Here we elucidate the structural and molecular determinant(s) of target specificity of histidine vs. lysine in the active site of SETD3. On the substrate-binding surface, the residues are diverse, reflecting the fact that the three enzymes act on three very distinct substrates—the large subunit of Rubisco by LSMT, RelA subunit of nuclear factor NFκB by SETD6, and actin by SETD3—with limited sequence similarity immediately surrounding the methylation target. To facilitate the methyl transfer reaction, SETD3 provides a local environment that promotes deprotonation of the target nitrogen N3 of histidine (and concomitant protonation of N1). Most (if not all) SAM-dependent MTases use the classic SN2 reaction mechanism, which requires the target nitrogen be in a deprotonated state.

Second, we incubated SETD3 with actin peptide in the presence of a molar excess of SAM (at pH 8.0) and crystallized the post-reactive product complex, i.e., the methylated histidine and SAH. The methyl group at the N3 position of methylhistidine is 3.2 Å away from the sulfur atom of SAH, where the transferable methyl group was attached before the reaction, and makes three weak C–H•••O hydrogen bonds, respectively, with the main chain carbonyl oxygen atoms of Thr252 and Asp274 as well as the hydroxyl oxygen of Tyr312. The methylated imidazole ring is perpendicular to the aromatic ring of Tyr312, and the nitrogen atom N1 is within H-bond distance from the side chain of Asn255. The current configuration of Asn255 appears to serve as a proton acceptor from the protonated N1 (N1–H•••O=C) of methylated H73; and to donate two protons to the main chain carbonyl oxygen atom of Ala268, and to a water molecule (numbered w2). The water (w2), in turn, forms three additional H-bonds with the main chain amide nitrogen atom of Ile270, one of the side chain carboxylate oxygen atoms of Asp274, and the main chain carbonyl oxygen atom of Arg253. This suggests that immediately after methyl transfer, the methylated histidine is positively charged with a protonated N1 (N1-H) and a methylated N3 (N3-CH3) and forms a cation–π interaction with Tyr312. The main difference between the pre-reactive and post-reactive complex structures is that the imidazole ring of methylated His73 rotated away from that of histidine.

>[2x]GPLGSMGKKSRVKTQKSGTGATATVSPKEILNLTSELLQKCSSPAPGPGKEWEEYVQIRTLVEKIRKKQKGLSVTFDGKREDYFPDLMKWASENGASVEGFEMVNFKEEGFGLRATRDIKAEELFLWVPRKLLMTVESAKNSVLGPLYSQDRILQAMGNIALAFHLLCERASPNSFWQPYIQTLPSEYDTPLYFEEDEVRYLQSTQAIHDVFSQYKNTARQYAYFYKVIQTHPHANKLPLKDSFTYEDYRWAVSSVMTRQNQIPTEDGSRVTLALIPLWDMCNHTNGLITTGYNLEDDRCECVALQDFRAGEQIYIFYGTRSNAEFVIHSGFFFDNNSHDRVKIKLGVSKSDRLYAMKAEVLARAGIPTSSVFALHFTEPPISAQLLAFLRVFCMTEEELKEHLLGDSAIDRIFTLGNSEFPVSWDNEVKLWTFLEDRASLLLKTYKTTIEEDKSVLKNHDLSVRAKMAIKLRLGEKEILEKAVKSAAVNREYYRQQMEEKAPLPKYEESNLGLLESSVGDSRLPLVLRNLEEEAGVQDALNIREAISKAKATENGLVNGENSIPNGTRSENESLNQESKRAVEDAKGSSSDSTAGVKE;>[2x]TLKYPIEHGIVTNWD> GCGACUCGGGGUGCCCUUCUGCGUGAAGGCUGAGAAAUACCCGUAU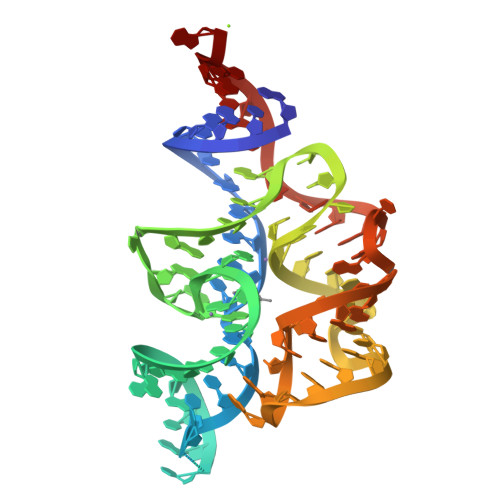CACCUGAUCUGGAUAAUGCCAGCGUAGGGAAGUCGCA> ALSEIETRHSEIIKLENSIRELHDMFMDM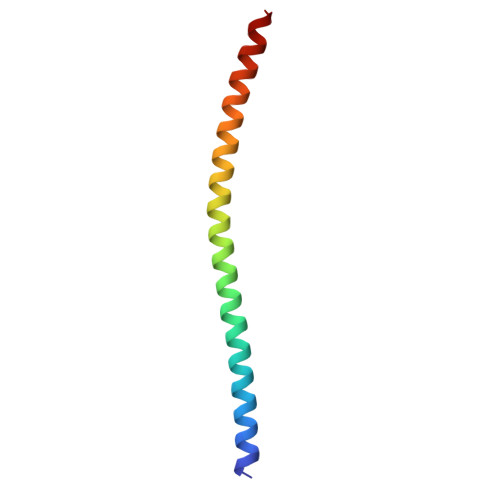AMLVESQGEMIDRIEYNVEHAVDYVERAVSDTKKAVK> YMW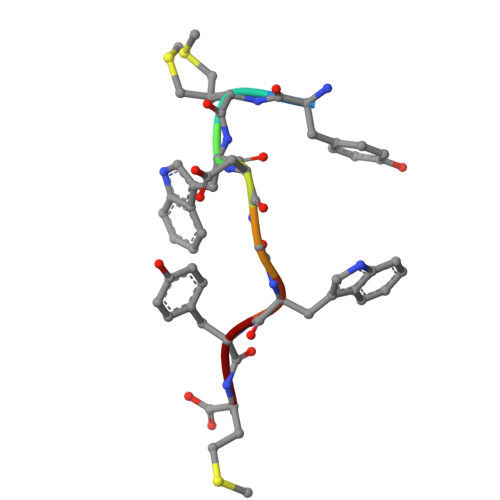DGWYM>[2x]GAMVKIIKKPKDVTALENATVAFEVSVSHDTVPVKWFHKSVEIKPSDKHRLVSERKVHKLMLQNISPSDAGEYTAVVGQLECKAKLFVETLHITKTMKNIEVPETKTASFECEVSHFNVPSMWLKNGVEIEMSEKFKIVVQGKLHQLIIMNTSTEDSAEYTFVCGNDQVSATLTV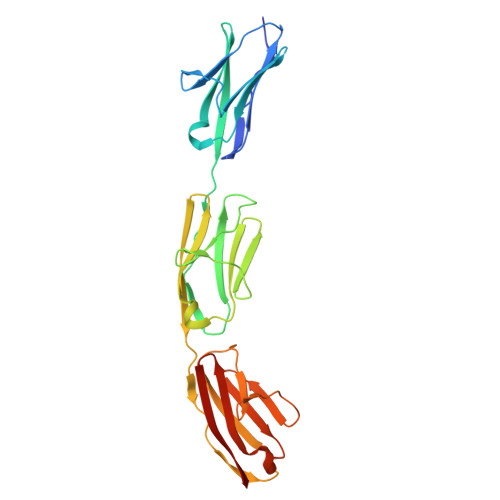TPIMITSMLKDINAEEKDTITFEVTVNYEGISYKWLKNGVEIKSTDKCQMRTKKLTHSLNIRNVHFGDAADYTFVAGKATSTATLYVVEA>MSLIPEIDAFLGCPTPDAWIEAALADQETLLIDHKNCEFKAASTALSLIAKYNTHLDLINMMSRLAREELVHHEQVLRLMKRRGVPLRPVSAGRYASGLRRLVRAHEPVKLVDTLVVGAFIEARSCERFAALVPHLDEELGRFYHGLLKSEARHYQGYLKLAHNYGDEADIARRVELVRAAEMELIQSPDQELRFHSGIPQALAA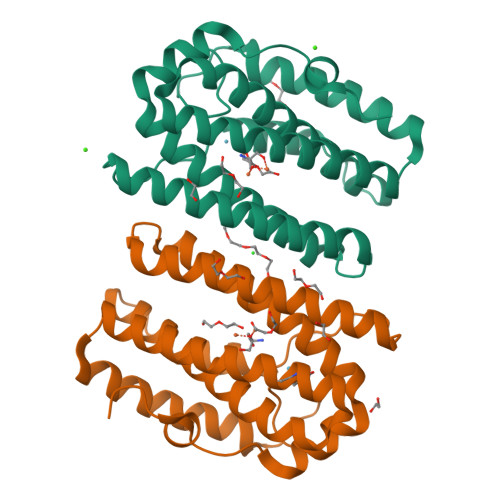[2x]>[8x]SGLLINQPKYSWLKELGLSEDNPGVYNGSWGGSGEVITSYCPANNEPIARVTQATLAEYEETVQKTREAWKMWADIPAPKRGEIVRQIGDALRKKIKVLGSLVSLEMGKIYVEGVGEVQEYVDVCDYAVGLSRMIGGPVLPSERPGHALIEQWNPVGLVGIITAFNFPVAVYGWNNAIALTCGNVCLWKGAPTTPLTSVAVTKIVAEVLEQNNLPGAICSMTCGGADIGTAMAKDERVDLLSFTGSTHVGKMVAMMVQERFGRK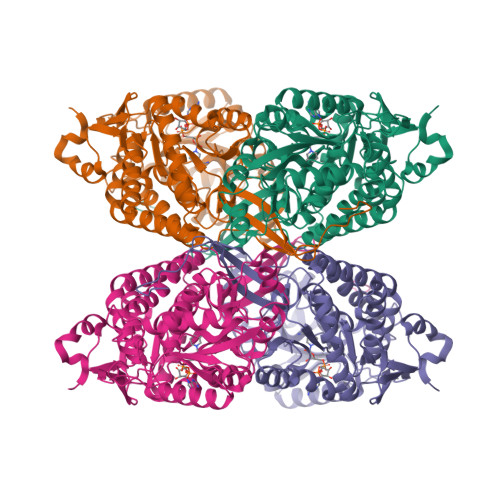LLELGGNNAIIVFEDADLNLVVPSAVFASVGTAGQRCTTTRRLMLHESVHDAVVERIAKAYKQVRIGDPWDPSTLYGPLHTKQAVDQYLAAIEQAKQQGGTLVCGGKVMDRPGNYVEPTIITGLAHDAPIVHTETFVPILYVLKFKTEEEAFAWNNEVQQGLSSSIFTKDLGRVFRWLGPKGSDCGIVNVNIPTSGAEIGGAFGGEKHTGGGRESGSDSWKQYMRRSTCTINYSKDLPLAQGIKFE>MSETPLLDELEKGPWPSFVKEIKKTAELMEKAAAEGKDVKMPKGARGLLKQLEISYKDKKTHWKHGGIVSVVGYGGGVIGRYSDLGEQIPEVEHFHTMRINQPSGWFYSTKALRGLCDVWEKWGSGLTNFHGSTGDII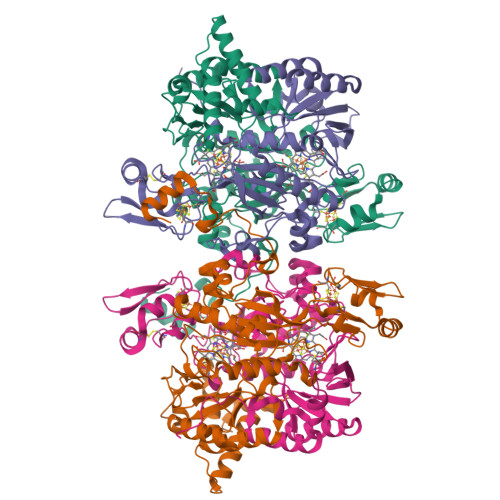FLGTRSEYLQPCFEDLGNLEIPFDIGGSGSDLRTPSACMGPALCEFACYDTLELCYDLTMTYQDELHRPMWPYKFKIKCAGCPNDCVASKARSDFAIIGTWKDDIKVDQEAVKEYASWMDIENEVVKLCPTGAIKWDGKELTIDNRECVRCMHCINKMPKALKPGDERGATILIGGKAPFVEGAVIGWVAVPFVEVEKPYDEIKEILEAIWDWWDEEGKFRERIGELIWRKGMREFLKVIGREADVRMVKAPRNNPFMFFEKDELKPSAYTEELKKRGMW[2x];>[2x]MVVEGVKTDFGPPYFRDLLHPVIAKNYGKWKYHEVVKPGVIKRVAESGDVIYVVRFGTPRLLSIYTVRELCDIADKYSDGYLRWTSRNNVEFFVTDESKIDDLINEVQERVGFPCGGTWDAVKGEYGLSNIVHTQGWIHCHTPAIDASGIVKAVMDELYEYFTDHKLPAMCRISLACCANMCGAVHASDIAIVGIHRTPPIPNDEAIRKTCEIPSTVAACPTGALKPDMKNKTIKVDVEKCMYCGNCYTMCPGMPLFDPENDGAAIMVGGKLSEARRMPELSKVVVPWVPNEPPRWPTLVKYVKQILEAWAANANKHERLIEWVDRIGWERFFELTGLEFTQHLIDDYRITPYFYSEFRASTQFKW>[2x]MAIPAFHPGELNVYSAPGDVADVSRALRLTGRRVMLVPTMGALHEGHLALVRAAKRVPGSVVVVSIFVNPMQFGAGGDLDAYPRTPDDDLAQLRAEGVEIAFTPTTAAMYPDGLRTTVQPG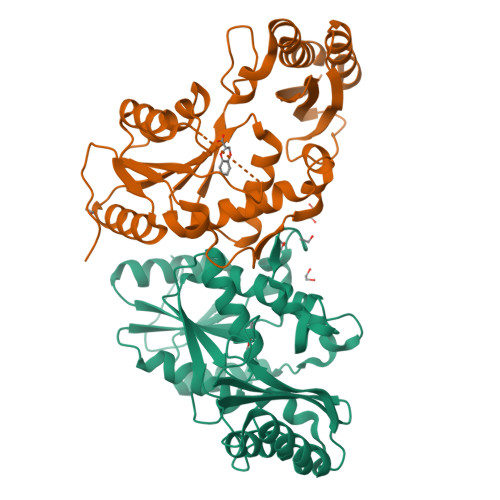PLAAELEGGPRPTHFAGVLTVVLKLLQIVRPDRVFFGEKDYQQLVLIRQLVADFNLDVAVVGVPTVREADGLAMSSRNRYLDPAQRAAAVALSAALTAAAHAATAGAQAALDAARAVLDAAPGVAVDYLELRDIGLGPMPLNGSGRLLVAARLGTTRLLDNIAIEIGTFAGTDRPDGYRA>GSHMMSTRPKISLIVAALQPSMGIGAKGSLPWRLKNEMKYFKDVTSKAKDGHINAVVMGRKTWELIPERFRPLAGRLNVILSRKNDDLIDSNGVYHFSSFDSVMKHLEKDSFRFKDMPLDKIFIIGGSQIYNLLILDSRVDNLLVTQVHFVGEDADKPQMDTFLDWDLSKWKRLEHDKLEQYVGLDVPRGLNEEGSYNYEYTMWEKAQ[2x]

Dihydrofolate reductase (DHFR) is a key and essential enzyme in the folate pathway that converts dihydrofolate (DHF) to tetrahydrofolate (THF) (Raimondi et al., 2019). This coenzyme is required for a variety of cellular processes, including the synthesis of purine involved in nucleic acid and amino-acid biosynthesis. The active site is located in a cleft formed by α-helix 1, α-helix 2, α-helix 4 and β-sheet 1, similar to CglDHFR and CalDHFR. As classified in E. coli DHFR, CauDHFR could also be designated to have two subdomains: the nucleotide subdomain, in which the NADPH sits, and the substrate-binding subdomain, which is predominantly formed by α-helix 1, α-helix 2 and β-sheet 1.

In order to reveal the binding modes of PYR and CYG, we obtained the ternary complexes CauDHFR–NADPH–PYR and CauDHDFR–NADPH–CYG. Interestingly, two CYG molecules are clearly observed as electron density in the DHF binding site of CauDHFR (named CYG1 and CYG2 here). CYG1 binds in an almost identical manner to PYR, but a secondary CYG2 also binds within the active site. For CYG2, the pyrimidine region interacts with the positively charged lip region, which is classically occupied by glutamate moieties, and the phenyl group occupies the apolar region that is classically occupied by the PABA moiety, stacked above the first CYG compound. The ternary complex with CYG only has slight conformational differences compared with the ternary complex with PYR, except for Phe65, which moves by 2.6 Å. This is most likely to be due to the steric clash that would arise in the ternary complex with CYG if it was in the same position as in the ternary complex with PYR. The Leu60 residue is shifted towards the NADPH molecule in both ternary complexes, being shifted 1.4 and 2.1 Å from the apoenzyme and holo­enzyme, respectively, with respect to CauDHFR–NADPH–PYR and 1.1 and 1.6 Å, respectively, with respect to CauDHFR–NADPH–CYG. The exception to this trend was CYG, with a significantly lower IC50 than would be expected from the thermal shift at 401 µM. This is a surprising result due to its largely similar crystal structure when compared with the CauDHFR–NADPH–PYR complex.> GSMVPPPENVRMNSVNFKNILQWESPAFAKGQLTFTAQYLSYRIFQDKCMQTTLTECDFSSLSKYGDHTLRVRAEFADEHSDWVQITFCPVDDTIIGPPGMQVEVLADSLHMRFLAPKIENEYETWTMKDMYNSWTYNVQYWKQGTDEKFQITPQYDFEVLRNLEPRTTYCVQVRGFLPDRNKAGEWSEPVCEQTTHDETVPSAAAHHHHHH;> RPRLAPPQNVTLLSQNFSVYLTWLPGLGNPQDVTYFVAYQSSPTRRRWREVEECAGTKELLCSMMCLKKQDLYNKFKGRVRTVSPSSKSPWVESEYLDYLFEVEPAPPVLVLTQTEEILSANATYQLPPCMPPLDLKYEVAFWKEGAGNKTLFPVTPHGQPVQITLQPAASEHHCLSARTIYTFSVPKYSKFSKPTCFLLEVPEANAAA;> GGGSGAAAPRRCLLSHYRSLEPRTLAAAKALRDRYEEEALSWGQRNCSFRPRRDPPRPSSCARLRHVARGIADAQAVLSGLHRSELLPGAGPILELLAAAGRDVAACLELARPGSSRKVPGAQKRRHKPRRADSPRCRKASVVFNLLRLLTWELRLAAHS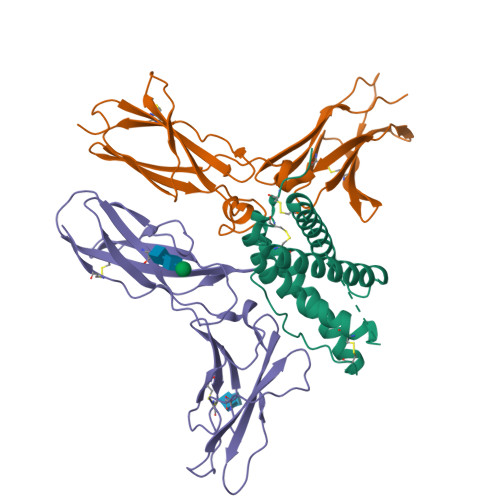GPCLAAAHHHHHHHH> ALFDRLGRVVRANLNDLVSKAEDPEKVLEQAVIDMQEDLVQLRQAVARTIAEEKRTEQRLNQDTQEAKKW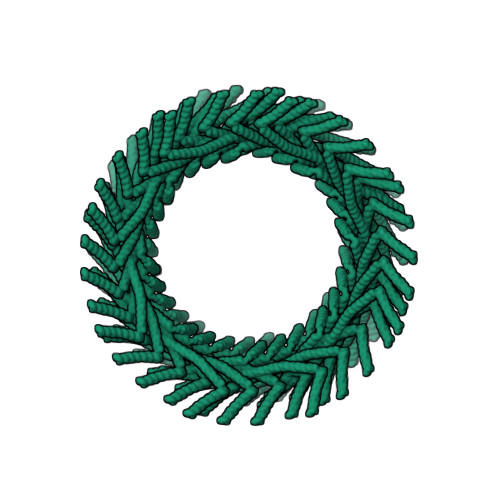EDRAKLALTNGEENLAREALARKKSLTDTAAAYQTQLAQQRTMSENLRRNLAALEAKISEAKTKKNMLQARAKAAKANAELQQTLGGLGTSSATSAFERMENKVLDMEATSQAAGELAGFGIENQFAQLEASSGVEDELAALKAS>SKYQCVKLNDGHFMPVLGFGTAAPAEVPKSKALEAVKLAIEAGFHHIDSAHVYNNEEQVGLAIRSKIADGSVKREDIFYTSKLWSNSHRPELVRPALERSLKNLQLDYVDLYLIHFPVSVKPGEEVIPKDENGKILFDTVDLCATWEAMEKCKDAGLAKSIGVSNFNHRLLEMILNKPGLKYKPVCNQVECHPYFNQRKLLDFCKSKDIVLVAYSALGSHREEPWVDPNSPVLLEDPVLCALAKKHKRTPALIALRYQLQRGVVVLA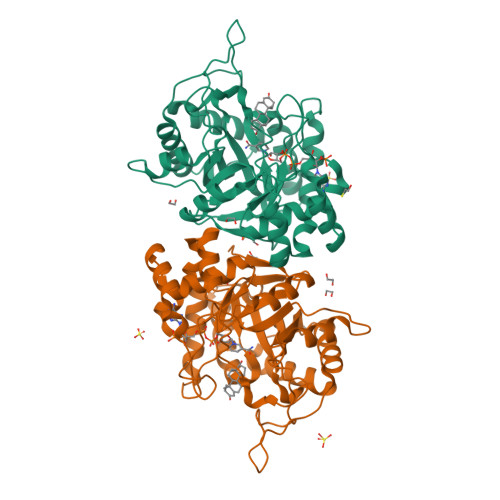KSYNEQRIRQNVQVFEFQLTSEEMKAIDGLNRNVRYLTLDIFAGPPNYPFSDEY[2x]>MSNAALATAPHALELDVHPVAGRIGAEIRGVKLSPDLDAATVEAIQAALVRHKVIFFRGQTHLDDQSQEGFAKLLGEPVAHPTVPVVDGTRYLLQLDGAQGQRANSWHTDVTFVEAYPKASILRSVVAPASGGDTVWANTAAAYQELPEPLRELADKLWAVHSNEYDYASLKPDIDPAK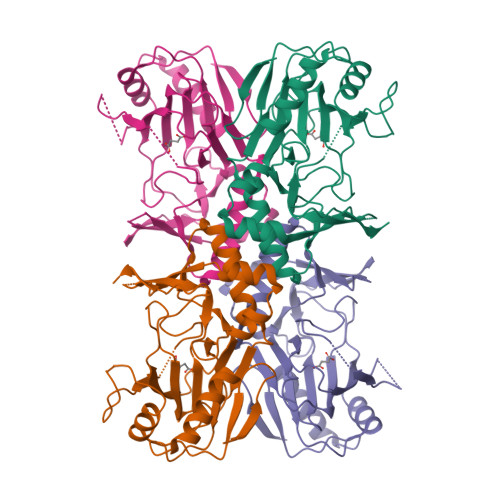LERHRKVFTSTVYETEHPVVRVHPISGERALQLGHFVKRIKGYSLADSQHLFAVLQGHVTRLENTVRWRWEAGDVAIWDNRATQHYAVDDYGTQPRIVRRVTLAGEVPVGVDGQLSRTTRKG[4x]>[2x]ASLGHPATFGRATHVVVRALPESLAQQALRRTKGDEVDFARAERQHQLYVGVLGSKLGLQVVQLPADESLPDCVFVEDVAVVCEETALITRPGAPSRRKEADMMKEALEKLQLNIVEMKDENA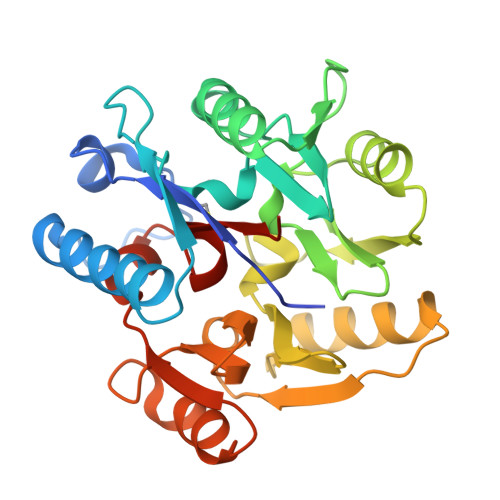TLDGGDVLFTGREFFVGLSKRTNQRGAEILADTFKDYAVSTVPVVDALHLKSFCSMAGPNLIAIGSSESAQKALKIMQQMSDHRYDKLTVPDDTAANCIYLNIPSKGHVLLHRTPEEYPESAKVYEKLKDHMLIPVSNSELEKVDGLLTCSSVLINKKVDS>[4x]MAAGVAAWLPFARAAAIGWMPVASGPMPAPPRQERKRTQDALIVLNVSGTRFQTWQDTLERYPDTLLGSSERDFFYHPETQQYFFDRDPDIFRHILNFYRTGKLHYPRHECISAYDEELAFFGLIPEIIGDCCYEEYKDRRRENAERLQDDADTDTAGESALPTMTARQRVWRAFENPHTSTMALVFYYVTGFFIAVSVIANVVETVPCGSSPGHIKELPCGERYAVAFFCLDTACVMIFTVEYLLRLAAAPSRYRFVRSVMSIIDVVAILPYYIGLVMTDNEDVSGAFVTLRVFRVFRIFKFSRHSQGLRILGYTLKSCASELGFLLFSLTMAIIIFATVMFYAEKGSSASKFTSIPAAFWYTIVTMTTLGYGDMVPKTIAGKIFGSICSLSGVLVIALPVPVIVSNFSRIYHQNQRADKRRAQKKARLARIRAAKSGSANAYMQSKRNGLLSNQLQSSEDEQAFVSKSGSSFETQHHHLLHCLEKTTNHEFVDEQVFEESCMEVATVNRPSSHSPSLSSQQGVTSTCCSRRHKKTFRIPNANVSGSHQGSIQELSTIQIRCVERTPLSNSRSSLNAKMEECVKLNCEQPYVTTAIISIPTPPVTTPEGDDRPESPEYSGGNIVRVSAL

Modulation of voltage-gated potassium (Kv) channels by auxiliary subunits is central to the physiological function of channels in the brain and heart. Native Kv4 tetrameric channels form macromolecular ternary complexes with two auxiliary β-subunits—intracellular Kv channel-interacting proteins (KChIPs) and transmembrane dipeptidyl peptidase-related proteins (DPPs)—to evoke rapidly activating and inactivating A-type currents, which prevent the backpropagation of action potentials. Here we report cryo-electron microscopy structures of the Kv4.2–DPP6S–KChIP1 dodecamer complex, the Kv4.2–KChIP1 and Kv4.2–DPP6S octamer complexes, and Kv4.2 alone. Thus, our data suggest that two distinct modes of modulation contribute in an additive manner to evoke A-type currents from the native Kv4 macromolecular complex.

We first determined the cryo-EM structures of human Kv4.2 alone and the Kv4.2–KChIP1 complex. The fourfold symmetrical structures of both Kv4.2 alone and the Kv4.2–KChIP1 complex were determined to an overall resolution of 2.9 Å by single-particle cryo-EM analysis with C4 symmetry imposed. The structure of Kv4.2 alone is compact with dimensions of around 75 Å × 75 Å × 100 Å and both N- and C-terminal regions (amino acids 1–39 and 437–630) are disordered. By contrast, the intracellular S6 helix bends at A419 in the structure of Kv4.2 alone, which results in a partial loss of interaction between the intracellular S6 helix and the T1–S1 linker, suggesting a key mechanism of Kv4 gating modulation by KChIPs. Moreover, while S6 gating helices adopt a more flexible conformation with weaker interaction with T1–S1 linkers in the structure of Kv4.2 alone, KChIP1 stabilizes these structures and enhances their interactions in the structure of Kv4.2–KChIP1.>MHHHHHHTSKIEQPRWASKDSAAGAASTPDEKIVLEFMDALTSNDAAKLIEYFAEDTMYQNMP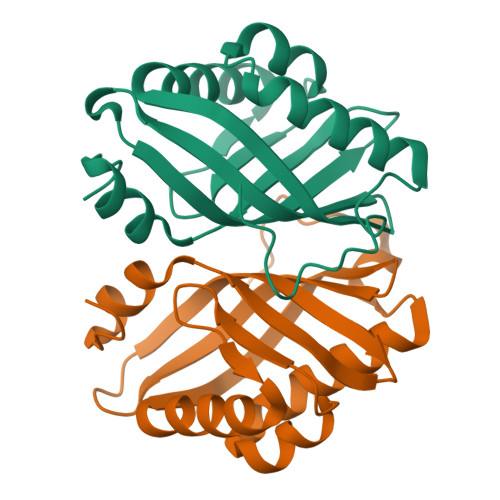LPPAYGRDAVEQTLAGLFTVMSYDAVETFHIGSSNGLVYTERVDVLRALPTGKSYNVSVLGVFQLTEGKITGWRDYFDLREFEEAVDLPLRG[4x]1-{2-[1-(aminomethyl)cyclohexyl]ethyl}-3-isoquinolin-6-ylurea | C19 H26 N4 O | 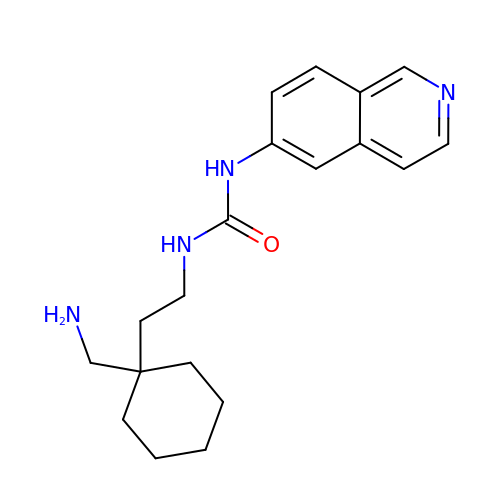NYAKHMNXWJGORW-UHFFFAOYSA-N> GPHMGGSMAEPVSPLKHFVLAKKAITAIFDQLLEFVTEGSHFVEATYKNPELDRIATEDDLVEMQGYKDKLSIIGEVLSRRHMKVAFFGRTSSGKSSVINAMLWDKVLPSGIGHITNCFLSVEGTDGDKAYLMTEGSDEKKSVKTVNQLAHALHMDKDLKAGCLVRVFWPKAKCALLRDDLVLVDSPGTDVTTELDSWIDKFCLDADVFVLVANSESTLMNTEKHFFHKVNERLSKPNIFILNNRWDASASEPEYMEDVRRQHMERCLHFLVEELKVVNALEAQNRIFFVSAKEVLSARKQKAQGMPESGVAL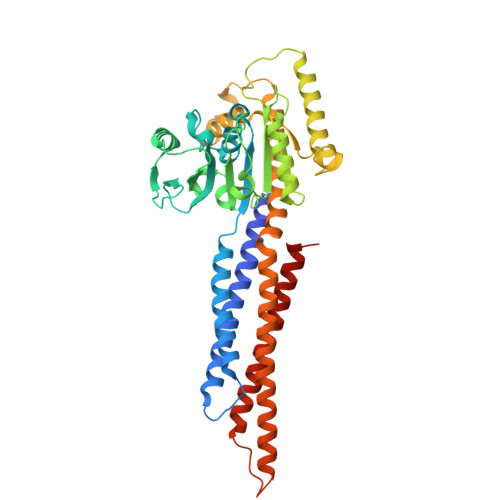AEGFHARLQEFQNFEQIFEECISQSAVKTKFEQHTIRAKQILATVKNIMDSVNLAAEDKSAASAASAASAASAAARLPKEIDQLEKIQNNSKLLRNKAVQLENELENFTKQFLPSSNEES> GSHMDSLRPKLSEEQQRIIAIL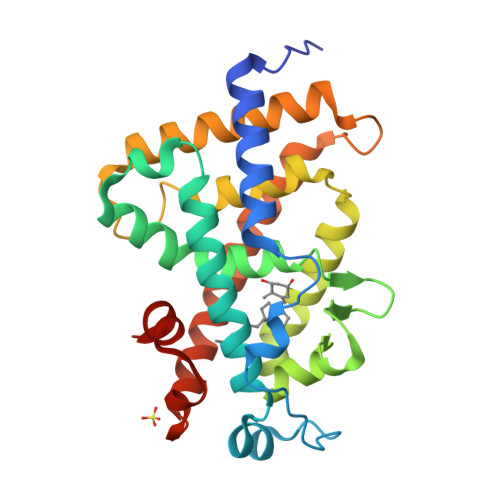LDAHHKTYDPTYSDFCQFRPPVRVNDGGGSVTLELSQLSMLPHLADLVSYSIQKVIGFAKMIPGFRDLTSEDQIVLLKSSAIEVIMLRSNESFTMDDMSWTCGNQDYKYRVSDVTKAGHSLELIEPLIKFQVGLKKLNLHEEEHVLLMAICIVSPDRPGVQDAALIEAIQDRLSNTLQTYIRCRHPPPGSHLLYAKMIQKLADLRSLNEEHSKQYRCLSFQPECSMKLTPLVLEVFGNEIS>[2x]MEEPEEPADSGQSLVPVYIYSPEYVSMCDSLAKIPKRASMVHSLIEAYALHKQMRIVKPKVASMEEMATFHTDAYLQHLQKVSQEGDDDHPDSIEYGLGYECPATEGI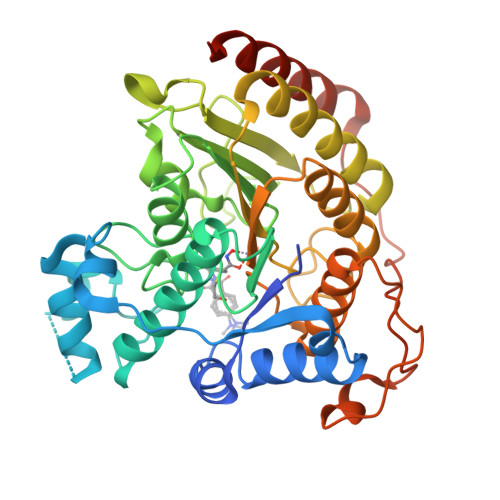FDYAAAIGGATITAAQCLIDGMCKVAINWSGGWHHAKKDEASGFCYLNDAVLGILRLRRKFERILYVDLDLHHGDGVEDAFSFTSKVMTVSLHKFSPGFFPGTGDVSDVGLGKGRYYSVNVPIQDGIQDEKYYQICESVLKEVYQAFNPKAVVLQLGADTIAGDPMCSFNMTPVGIGKCLKYILQWQLATLILGGGGYNLANTARCWTYLTGVILGKTLSSEIPDHEFFTAYGPDYVLEITPSCRPDRNEPHRIQQILNYIKGNLKHVVIEGRSHHHHHH>KMKLYNFWRSGTSHRLRIALNLKGVPYEYLAVHLGKEEHLKDAFKALNPQQLVPALDTGAQVLIQSPAIIEWLEEQYPTPALLPADADGRQRVRALAAIVGCDIHPINNRRILEYLRKTFGADEAAINAWCGTWISAGFDAYEALLAVDPKRGRYS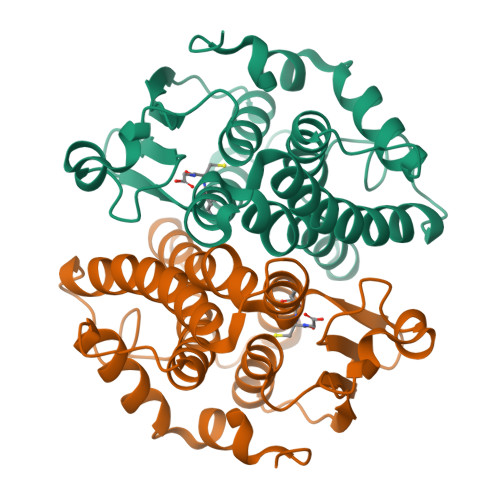FGDTPTLADCYLVPQVESARRFQVDLTPYPLIRAVDAACGELDAFRRAAPAAQPDSA[2x]> ASLTEIEHLVQSVCKSYRETCQLRLEDLLRQRSNIFSREEVTGYQRKSMWEMWERCAHHLTEAIQYVVEFAKRLSGFMELCQNDQIVLLKAGAMEVVLVRMCRAYNADN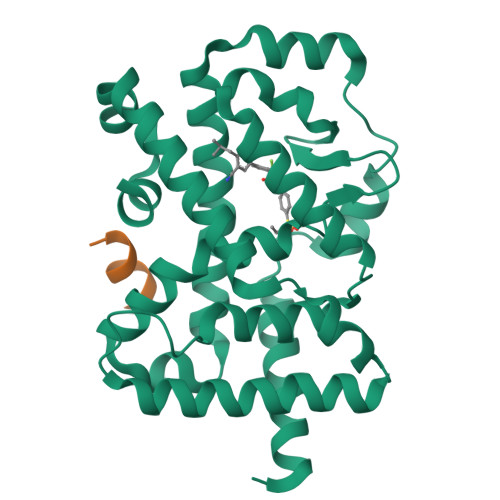RTVFFEGKYGGMELFRALGCSELISSIFDFSHSLSALHFSEDEIALYTALVLINAHRPGLQEKRKVEQLQYNLELAFHHHLCKTHRQSILAKLPPKGKLRSLCSQHVERLQIFQHLHPIVVQAAFPPLYKELFSTE;> KILHRLLQ> MASLNLAPEELKQLELLRNRFAQLQSSLTSLAGNLIRTEPLPTYESLQASASILQQNLRSIQELMTENSDIFKRIAIHPSTNFP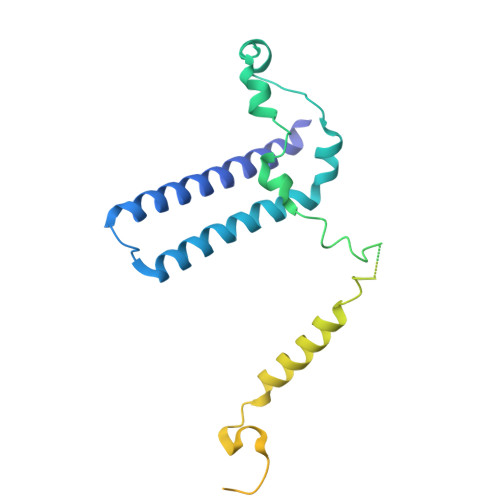GRTQEHMLLQLLRKKLEPEVESWVEEARETARAAGIDVSKLSGPGGGAPTRGMNGYGDDDEYGLDDEDEGVPSDPFNEQWADMLETFQHSLHHYVTVQLKKQYTVEEQEMGIENVRTGLKRELGDEDEDEDEDEEEEEEGVAGVAGGAASQGAGAGTAGAAAKKPVIQPEYLFWLAARGDTRVSRNIEFEAMRKVAQTAKRPAPPR6-(4-fluorophenyl)quinazolin-8-ol | C14 H9 F N2 O | 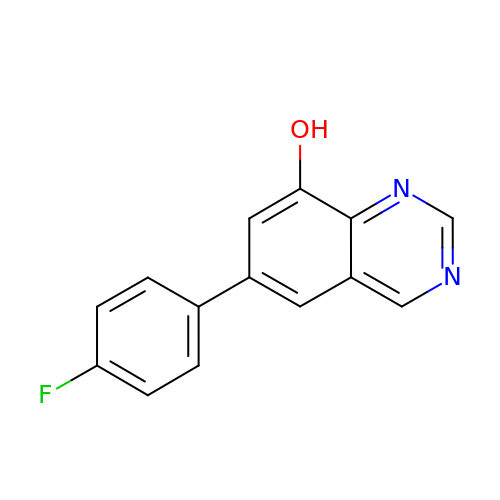QTUPQWZWXNDRNS-UHFFFAOYSA-N>MDSKQQCVKLNDGHFMPVLGFGTYAPPEVPRSKALEVTKLAIEAGFRHIDSAHLYNNEEQVGLAIRSKIADGSVKREDIFYTSKLWSTFHRPE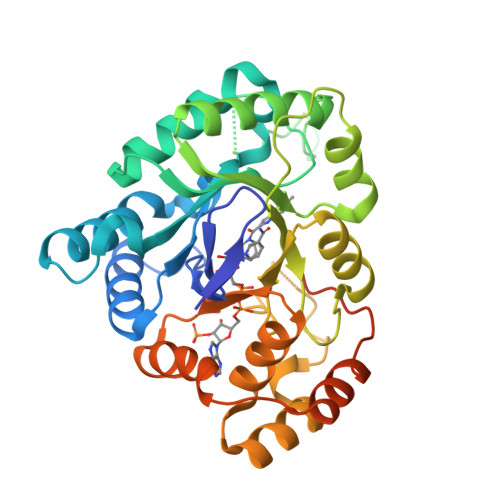LVRPALENSLKKAQLDYVDLYLIHSPMSLKPGEELSPTDENGKVIFDIVDLCTTWEAMEKCKDAGLAKSIGVSNFNRRQLEMILNKPGLKYKPVCNQVECHPYFNRSKLLDFCKSKDIVLVAYSALGSQRDKRWVDPNSPVLLEDPVLCALAKKHKRTPALIALRYQLQRGVVVLAKSYNEQRIRQNVQVFEFQLTAEDMKAIDGLDRNLHYFNSDSFASHPNYPYSDEYLEHHHHHH[2x]>ATPHINAEMGDFADVVLMPGDPLRAKYIAET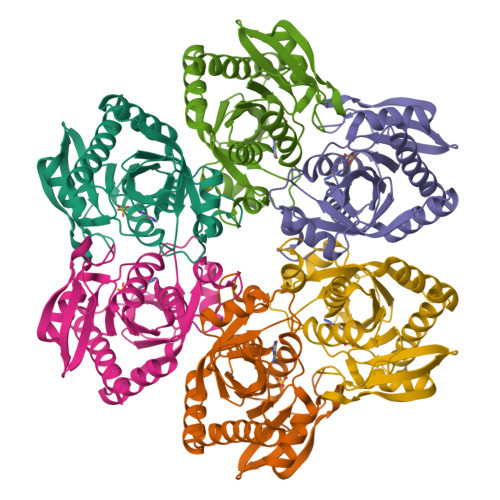FLEDAREVNNVRGMLGFTGTYKGRKISVMGHGMGIPSCSIYTKELITDFGVKKIIRVGSCGAVLPHVKLRDVVIGMGACTDSKVNRIRFKDHDFAAIADFDMVRNAVDAAKALGIDARVGNLFSADLFYSPDGEMFDVMEKYGILGVEMEAAGIYGVAAEFGAKALTICTVSDHIRTHEQTTAAERQTTFNDMIKIALESVLLGDK[3x]>MRRLLFLSLAGLWLFSPAAAAQLPGLISQPLAGGGQSWSLSVQTLVFITSLTFLPAILLMMTSFTRIIIVFGLLRNALGTPSAPPNQVLLGLALFLTFFIMSPVIDKIYVDAYQPFSEQKISMQEALDKGAQPLRAFMLRQTREADLALFARLANSGPLQGPEAVPMRILLPAYVTSELKTAFQIGFTIFIPFLIIDLVIASVLMALGMMMVPPATIALPFKLMLFVLVDGWQLLMGSLAQSFYS[5x];> MIQVTSEQWLYWLHLYFWPLLRVLALISTAPILSERAIPKRVKLGLGIMITLVIAPSLPANDTPLFSIAALWLAMQQILIGIALGFTMQFAFAAVRTAGEFIGLQMGLSFATFVDPGSHLNMPVLARIMDMLAMLLFLTFNGHLWLISLLVDTFHTLPIGSNPVNSNAFMALARAGGLIFLNGLMLALPVITLLLTLNLALGLLNRMAPQLSIFVIGFPLTLTVGIMLMAALMPLIAPFCEHLFSEIFNLLADIVSEMPINNNPHHHHHHHHHH;>[4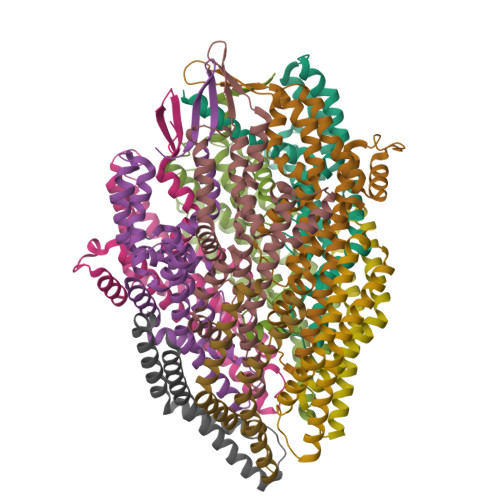x]MTPESVMMMGTEAMKVALALAAPLLLVALITGLIISILQAATQINEMTLSFIPKIVAVFIAIIVAGPWMLNLLLDYVRTLFSNLPYIIG L-arginine oxidase (AROD, EC 1.4.3.25) is an oxidoreductase that catalyses the deamination of L-arginine, with flavin adenine dinucleotide (FAD) as a cofactor. Recently identified AROD from Pseudomonas sp. TPU 7192 (PT-AROD) demonstrates high selectivity for L-arginine. This enzyme is useful for accurate assays of L-arginine in biological samples.

Here, we report the structure of PT-AROD at a resolution of 2.3 Å by cryo-electron microscopy. PT-AROD adopts an octameric structure with D4 symmetry, which is consistent with its molecular weight in solution, estimated by mass photometry. Comparative analysis of this structure with that determined using X-ray crystallography reveals open and closed forms of the lid-like loop at the entrance to the substrate pocket.

> MHHHHHHMSQTQPLDVAIIGGGVSGTYSAWRLQEAQGDHQRIQLFEYSDRIGGRLFSINLPGLPNVVAEVGGMRWMPATKDNTGGHVMVDKLVGELKLESKNFPMGSNLPDKDPVGAKDNLFYLRGERFRLRDFTEAPDKIPYKLAWSERGYGPEDLQVKVMHNIYPGFDKLSLAEQMQVKVFGKEIWRYGFWDLLYRVLSNEGYQFMKDAGGYEANVANASAVTQLPATEYSDKTVFLALKKGFQALPLTLAKRFAEVPGGLIAGEQRIRMNRRLASVQFSDDTEYPYRLHFQATRTVDGKTSDVPGAEEIIHARQVILALPRRSLELIQSPLFDDPWLKENIDSVLVQSAFKLFLAYEQPWWRSQGLVAGRSVTDLPIRQCYYMGTECEQDGGEKTLNSLLMASYNDIGTVPFWKGLEDGAPFEGYQPKSLQGRIDANEVVPKMQYQISEEMVRIAQRQVTSLHDQIELPAPYSAVYHAWDADPFGGGWHEWKANYRLDLIIQRMRHPVQEQEVYIVGEAYSYGQGWVEGALTTAESTLQDFFGLPRPAWLPEAYQLLPAPAPVDIDNPPALACTDCKKTLTEVTEFAYTGIKA> MSGSMKEEIKRLAEE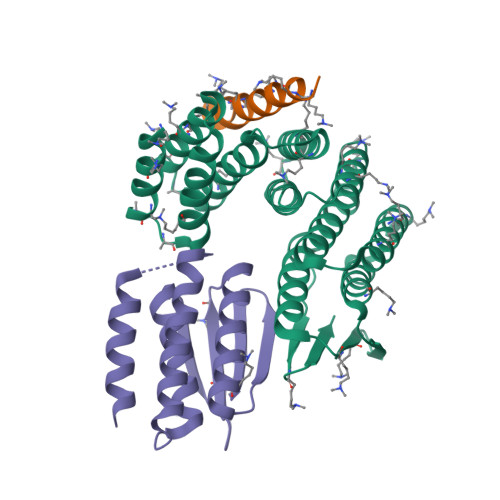LKEKTKNEEIKRLAEEAAELAERSDDPEVLEVVKKALEEALKSKNEEKIELLLLVAVLVAEAGSVDAVEEKLEIALLALKLAEESKDPRIIRGALRAAIAALRSDDPLALKTVKEALERARASKDERLIRAILAAAYAFALLAVAGASAERLKEAEAIVKELIAAAEKGASPQELVLLVIEMMVKGMGVTMETHRSGNEVKVVIKGLHESQQEVLLEAVLFAAELMGVRVRIRFKGDTVTIVV;> RKKELAKEVIETAKKLIEKLAKEE;> EEAVRRRFEELLREALAFRERTGGRRETLEHAVRLARELAEFAASHPEFNRQEAVLLAIELMVRAMGVTMETHRSGNEVKVVIKGLNIDEQVALYRAVRETSKIMGVETEIEVEGDTQTIVV> RPGGDTIF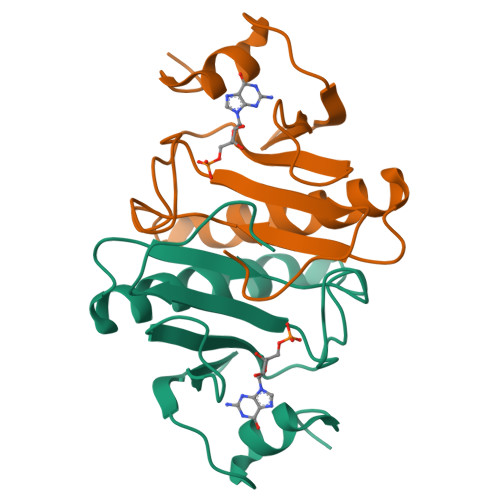GKIIRKEIPAKIIFEDDQCLAFHDISPQAPTHFLVIPKKHISQISAAEDADESLLGHLMIVGKKCAADLGLKKGYRMVVNEGSDGGQSVYHVHLHVLGGRQMNWPPG The zinc-uptake protein ZnuD is expressed under zinc-limiting conditions and was originally discovered in Neisseria meningitidis, where its expression is under the control of a zinc-sensing transcriptional factor, Zur14. ZnuD is an 82 kDa outer-membrane protein predicted to be a member of the TonB-dependent receptor (TbdR) family, requiring the mechanical energy derived from the TonB/ExbB/ExbD inner-membrane complex to couple nutrient uptake to the proton gradient across the inner-membrane. Characteristic of other TbdR family members, ZnuD consists of an amino-terminal plug domain (residues 1 to 147) obstructing the lumen of its own carboxy-terminal pore-forming domain (residues 148 to 734). Combined with molecular dynamic (MD) simulations, our structural findings suggest that ZnuD acquires free zinc ions using a series of binding sites that move zinc across the outer-membrane through a transient pore that requires TonB activation.

To elucidate the metal transportation mechanism, we attempted to capture ‘snapshots' of ZnuD in multiple translocation binding-states through co-crystallization and by soaking ZnuD with zinc or cadmium ions. The transition metal cadmium, which mimics and competes with zinc-binding sites in proteins, was a critical tool to stabilize and identify two additional binding sites. Indeed, all three ZnuD intermediate structures presented in this study contain a zinc ion buried in a high-affinity zinc-binding pocket. The metal ion captured within the high-affinity binding site is coordinated by four conserved residues (Asp-99, His-100, Glu-340 and His-499) located in a buried pocket that is sealed by the plug-apical loop and extracellular loop 6. The presence of zinc modulates the dynamic flexibility of the external loops by remodelling an α-helical segment into a pair of β-strand motifs. In addition, on binding its zinc ions on peripheral sites, the immunogenic loop 3 undergoes major conformational changes resulting in a switch between rigid (β-strand pairs) and flexible (α-helix) conformations. Our three structures illustrate that ZnuD undergoes drastic surface variations upon substrate binding to peripheral zinc-binding sites.

> MAHHHHHHLVPRGSHETEQSVDLETVSVVGKSRPRATSGLLHTSTASDKIISGDTLRQKAVNLGDALDGVPGIHASQYGGGASAPVIRGQTGRRIKVLNHHGETGDMADFSPDHAIMVDTALSQQVEILRGPVTLLYSSGNVAGLVDVADGKIPEKMPENGVSGELGLRLSSGNLEKLTSGGINIGLGKNFVLHTEGLYRKSGDYAVPRYRNLKRLPDSHADSQTGSIGLSWVGEKGFIGVAYSDRRDQYGLPAHSHEYDDCHADIIWQKSLINKRYLQLYPHLLTEEDIDYDNPGLSCGFHDDDNAHAHTHSGRPWIDLRNKRYELRAEWKQPFPGFEALRVHLNRNDYRHDEKAGDAVENFFNNQTQNARIELRHQPIGRLKGSWGVQYLQQKSSALSAISEAVKQPMLLDNKVQHYSFFGVEQANWDNFTLEGGVRVEKQKASIQYDKALIDRENYYNHPLPDLGAHRQTARSFALSGNWYFTPQHKLSLTASHQERLPSTQELYAHGKHVATNTFEVGNKHLNKERSNNIELALGYEGDRWQYNLALYRNRFGNYIYAQTLNDGRGPKSIEDDSEMKLVRYNQSGADFYGAEGEIYFKPTPRYRIGVSGDYVRGRLKNLPSLPGREDAYGNRPFIAQDDQNAPRVPAARLGFHLKASLTDRIDANLDYYRVFAQNKLARYETRTPGHHMLNLGANYRRNTRYGEWNWYVKADNLLNQSVYAHSSFLSDTPQMGRSFTGGVNVKF>MEGSVNGSQRGNGSQRERVPEPGAGPTTDLLRDSRSLRGIFSSFATGVTVVTVGGDSPHAMTANSFTSVSLDPPLILVCVECDAAMHGSLLEVGSFGVSVLAADQQHVALLYANRWRPRDPTQFDRPGWARGARTGAPLARGALAWFECALWRAYDAGDHSIFVGRLLTAERHDRRDALVYHSGQFRGLPDRAP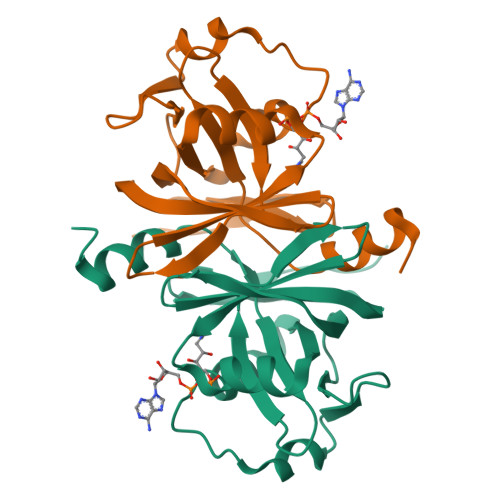VE[8x]Splicing modulators alter the splicing patterns in cells by binding to the U2 snRNP (small nuclear ribonucleoprotein)—a complex chaperoning the selection of branch and 3′ splice sites. The U2 snRNP has a bipartite organization, exhibiting a smaller U2 3′ module and a larger U2 5′ module. The latter contains the heptameric SF3B complex, whose core subunit SF3B1 is recurrently mutated in cancers. In this work, by employing FR901464 analogs as molecular tools to dissect the splicing pathway, we elucidate how spliceostatins/sudemycins interfere with prespliceosome assembly and splicing commitment by covalent coupling to a reactive zinc finger of PHF5A.

We have engineered a variant of the human SF3B core that lacks the β-propeller BPB domain of SF3B3 (SF3BΔBPB). The complex formed crystals in two alternative space-groups, belonging to the orthorhombic and trigonal symmetry systems. Our best orthorhombic crystals diffracted X-rays to a resolution of 2.3 Å, while diffraction data for the trigonal form was limited to ~3.0 Å. The distal half of the SSA molecule (C11-C15) establishes hydrophobic contacts and hydrogen bonds with the hinged pocket. The proximal half of SSA (atoms C1–C10) extends away from the tunnel towards one of the zinc fingers of PHF5A (i.e., Znf1). Its epoxy-tetrahydropyran group is recognized by a hydrogen bond network, involving SF3B1 and PHF5A residues and several solvent molecules in the binding pocket. Strikingly, SSA’s epoxide group resides close to C26-PHF5A—one of the four cysteine residues of PHF5A’s Znf1 zinc cluster. The electron density is continuous between C26-PHF5A and the epoxide group, while absent between C26-PHF5A and Znf1’s zinc ion, indicating an intermolecular covalent bond between SSA and C26-PHF5A. Notably, a thiocyanate ion replaces the water molecule at Znf1 in the orthorhombic SF3BΔBPB-crystals that grow in 200 mM potassium thiocyanate. The 2.3 Å resolution of these crystals enables visualization of thiocyanate’s distinctive elongated shape next to the zinc atom.

> GAEFKGLRRHMFLYNLTLQRATGISFAIHGNFSGTKQQEIVVSRGKILELLRPDPNTGKVHTLLTVEVFGVIRSLMAFRLTGGTKDYIVVGSDSGRIVILEYQPSKNMFEKIHQETFGKSGCRRIVPGQFLAVDPKGRAVMISAIEKQKLVYILNRDAAARLTISSPLEAHKANTLVYHVVGVDVGFENPMFACLEMDYEEADNDPTGEAAANTQQTLTFYELDLGLNHVVRKYSEPLEEHGNFLITVPGGSDGPSGVLICSENYITYKNFGDQPDIRCPIPRRRNDLDDPERGMIFVCSATHKTKSMFFFLAQTEQGDIFKITLETDEDMVTEIRLKYFDTVPVAAAMCVLKTGFLFVASEFGNHYLYQIAHLGDDDEEPEFSSAMPLEEGDTFFFQPRPLKNLVLVDELDSLSPILFCQIADLANEDTPQLYVACGRGPRSSLRVLRHGLGGNGNSGEKLGAVFNQVAFPLQYTPRKFVIHPESNNLIIIETDHNAYTEATKAQRKQQMAEEMVEAAGEDERELAAEMAAAFLNENLPESIFGAPKAGNGQWASVIRVMNPIQGNTLDLVQLEQNEAAFSVAVCRFSNTGEDWYVLVGVAKDLILNPRSVAGGFVYTYKLVNNGEKLEFLHKTPVEEVPAAIAPFQGRVLIGVGKLLRVYDLGKKKLLRKCENKHIANYISGIQTIGHRVIVSDVQESFIWVRYKRNENQLIIFADDTYPRWVTTASLLDYDTVAGADKFGNICVVRLPPNTNDEVDSQKAEVIMNYHVGETVLSLQKTTLIPGGSESLVYTTLSGGIGILVPFTSHEDHDFFQHVEMHLRSEHPPLCGRDHLSFRSYYFPVKNVIDGDLCEQFNSMEPNKQKNVSEELDRTPPEVSKKLEDIRTRYAQLEQNEAAF;> MTDRYTIHSQLEHLQSKYIGTGHADTTKWEWLVNQHRDSYCSYMGHFDLLNYFAIAENESKARVRFNLMEKMLQPCGPPADKPEEN;> MKSVNDQPSGNLPFLKPDDIQYFDKLLVDVDESTLSPEEQKERKIMKLLLKIKNGTPPMRKAALRQITDKAREFGAGPLFNQILPLLMSPTLEDQERHLLVKVIDRILYKLDDLVRPYVHKILVVIEPLLIDEDYYARVEGREIISNLAKAAGLATMISTMRPDIDNMDEYVRNTTARAFAVVASALGIPSLLPFLKAVCKSKKSWQARHTGIKIVQQIAILMGCAILPHLRSLVEIIEHGLVDEQQKVRTISALAIAALAEAATPYGIESFDSVLKPLWKGIRQHRGKGLAAFLKAIGYLIPLMDAEYANYYTREVMLILIREFQSPDEEMKKIVLKVVKQCCGTDGVEANYIKTEILPPFFKHFWQHRMALDRRNYRQLVDTTVELANKVGAAEIISRIVDDLKDEAEQYRKMVMETIEKIMGNLGAADIDHKLEEQLIDGILYAFQEQTTEDSVMLNGFGTVVNALGKRVKPYLPQICGTVLWRLNNKSAKVRQQAADLISRTAVVMKTCQEEKLMGHLGVVLYEYLGEEYPEVLGSILGALKAIVNVIGMHKMTPPIKDLLPRLTPILKNRHEKVQENCIDLVGRIADRGAEYVSAREWMRICFELLELLKAHKKAIRRATVNTFGYIAKAIGPHDVLATLLNNLKVQERQNRVCTTVAIAIVAETCSPFTVLPALMNEYRVPELNVQNGVLKSLSFLFEYIGEMGKDYIYAVTPLLEDALMDRDLVHRQTASAVVQHMSLGVYGFGCEDSLNHLLNYVWPNVFETSPHVIQAVMGALEGLRVAIGPCRMLQYCLQGLFHPARKVRDVYWKIYNSIYIGSQDALIAHYPRIYNDDKNTYIRYELDYIL;> GPLGSPGSRAMAKHHPDLIFCRKQAGVAIGRLCEKCDGKCVICDSYVRPCTLVRICDECNYGSYQGRCVICGGPGVSDAYYCKECTIQEKDRDGCPKIVNLGSSKTDL>[2x]DAMDITVSIPPQQYFLEKIGGDLVRVSVLVPGNNDPHTYEPKPQQLAALSEAEAYVLIGLGFEQPWLEKLKAANANMKLIDSAQGITPLEMEKHDHSHGEEEGHDDHSHDG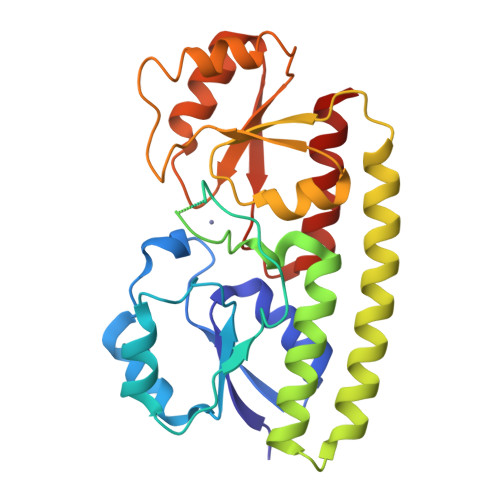HDHGSESEKEKAKGALMVADPHIWLSPTLVKRQATTIAKELAELDPDNRDQYEANLAAFLAELERLNQELGQILQPLPQRKFIVFHPSWAYFARDYNLVQIPIEVEGQEPSAQELKQLIDTAKENNLTMVFGETQFSTKSSEAIAAEIGAGVELLDPLAADWSSNLKAVAQKIANANSAQ B. burgdorferi dispenses with the use of thiamin as a cofactor and relies on lactate dehydrogenase (BbLDH) to convert pyruvate to lactate for balancing NADH/NAD+ ratios. BB_0087 (BbLDH) comprises 316 residues and is annotated as the sole LDH in the genome of B. burgdorferi. Biochemical analyses reveal that BbLDH behaves similarly to other LDHs, interconverting pyruvate and lactate through oxidation/reduction of NADH/NAD+. BbLDH forms a homo-tetramer or a dimer of dimers, wherein each monomer comprises eight α-helices and five β-strands and contains binding sites for oxamate, NADH, and FBP.

The crystal structures of BbLDH with and without FBP were determined via X-ray crystallography to a resolution of 2.1 Å. Both structures were determined in the presence of NADH and the pyruvate analog oxamate (OXA). Interestingly, FBP binding does not change the overall structure of the BbLDH tetramer to any appreciable extent, with the FBP-bound tetramer superimposing on the apo-tetramer with an RMSD of 0.230 Å. Within the BbLDH tetramer, the four NADH/oxamate binding sites (one per subunit) are highly similar, as are the two FBP binding sites (one per dimer), with the only major difference being the relative position of the Gln85-Arg91 loop adjacent to the NADH/oxamate binding site. In addition, mutation of the key residue His171 to Ala completely abolished the FBP-mediated allosteric activation on BB_0087 as this residue forms eight hydrogen bonds with FBP (four on each chain) to stabilize the interaction between BbLDH and FBP. LDH subunit conformations can be classified as either relaxed (R)- or taut (T)-state, with the allosteric regulator FBP favoring the R-state. However, in BbLDH, FBP does not result in the tetramer-wide conformational conversion from the low-substrate affinity T-state to the high-substrate-affinity R-state, largely because the FBP-minus structures are already in a primarily R-state conformation. The structural insensitivity to FPB may be a result of the high oxamate concentrations used in both crystallization conditions, which will favor the R-state conformation. The two FBP-bound BbLDH dimers within the tetramer are practically identical, except for the relative position of the A-loop. Hence, in BbLDH, the A-loop is conformationally variable regardless of the presence of FBP.

>[4x]MLKSNKVVLIGAGGVGSSFAYALTIDNSLVHELVIIDVNENKAKGEVMDLNHGQMFLKKNINVLFGTYKDCANADIVVITAGLNQKPGETRLDLVDKNSKIFKDIITNVVSSGFDGIFVVASNPVDIMTYVTMKYSKFPIHKVIGTGTILDTSRLRYFLSDHFNVNTQNIHSYIMGEHGDSSFATWDETKIAMKPLSEYLAEGKITELELDEIHKKVVNAAYEVIKLKGATYYAIGLGIKNIVNAIIGDQNVILPISSYINGQYGGLIKDIYIGAPAIVCKEGVKEVLNFKISPKELDKFNSSANQLKSYIDKM>[2x]PSVYDAAAQLTADVKKD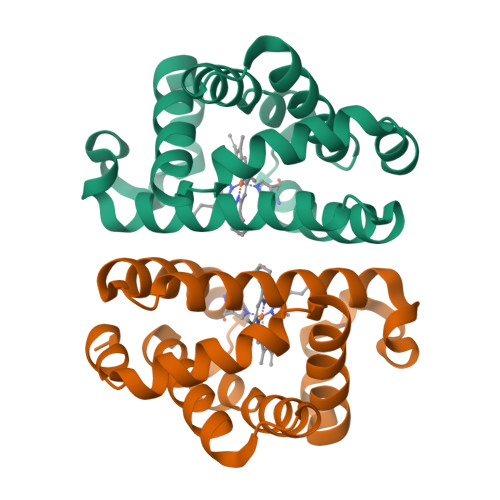LRDSWKVIGSDKKGNGVAFMTTLFADNQETIGYFKRLGDVSQGMANDKLRGHSITLMYALQNFIDQLDNPDDLVCVVEKFAVNHITRKISAAEFGKINGPIKKVLASKNFGDKYANAWAKLVAVVQAAL>[21x]MITNNLVPTVIEKTAGGERAFDIYSRLLKERIVFLNGEVNDHSANLVIAQLLFLESEDPDKDIYFYINSPGGMVTAGMGVYDTMQFIKPDVSTICIGLAASMGSLLLAGGAKGKRYSLPSSQIMIHQPLGGFRGQASDIEIHAKNILRIKDRLNKVLAHHTGQDLETIVKDTDRDNFMMADEAKAYGLIDHVIESREAIIK

Caseinolytic proteases are large oligomeric assemblies responsible for maintaining protein homeostasis in bacteria and in so doing influence a wide range of biological processes. The functional assembly involves three chaperones together with the oligomeric caseinolytic protease catalytic subunit P (ClpP). This protease represents a potential target for therapeutic intervention in pathogenic bacteria. Here, we detail an efficient protocol for production of recombinant ClpP from Francisella tularensis, and the structural characterization of three crystal forms which grow under similar conditions.

One crystal form reveals a compressed state of the ClpP tetradecamer and two forms an open state. A comparison of the two types of structure infers that differences at the enzyme active site result from a conformational change involving a highly localized disorder‐order transition of a β‐strand α‐helix combination. This transition occurs at a subunit‐subunit interface.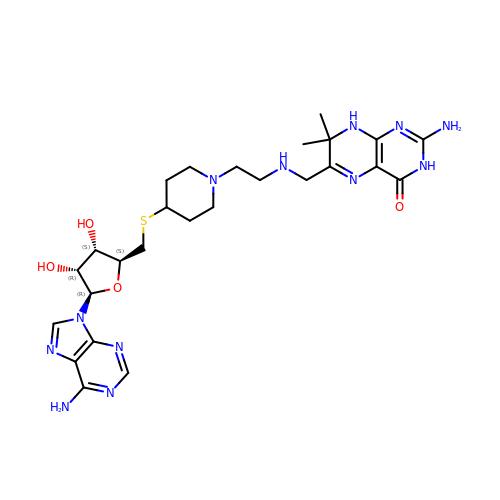5'-S-[1-(2-{[(2-amino-7,7-dimethyl-4-oxo-3,4,7,8-tetrahydropteridin-6-yl)methyl]amino}ethyl)piperidin-4-yl]-5'-thioadenosine | C26 H38 N12 O4 S | SQZWJXDKQKNJEE-KYKAGHOCSA-N>GAMGKDSNESKKHKKEKRKGKVENLLVAINNLKNPTKPAAGKNKANSKASKQKNNPNANANNAPK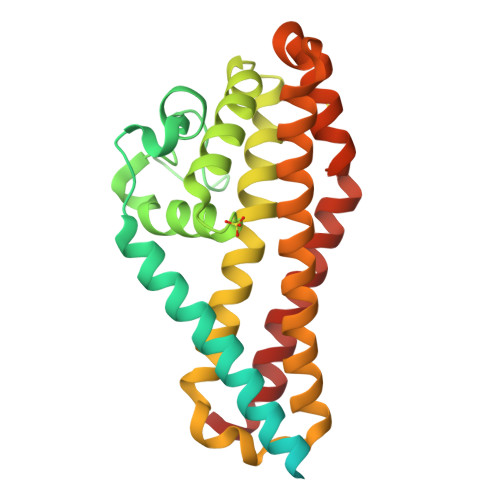KILDPEVAKLIQKILDRSENIIQISEMDSSRGEPNDQFGMRAEIFSKIFFNANSTVHFDSHEYTEERRMLYTSLNFNEGKIFNLGQILSKLSQDSNYRGLVKETLINRGFSIQLAMEEISAKILNVKDKLQQLNKPNLETLYNDFEKLTSLKEKWLKDTDDLIDEYNTNPDLQTDVSKLNDTLRSKNSRAQFANIHDIILDLVNTTTNILAPIQ[2x]>[2x]MYVCLCQGVTDNQI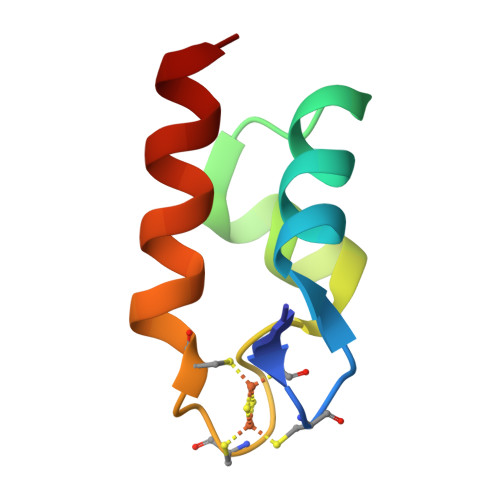RDAIYEGCCSYREVREATGVGTQCGKCASLAKQVVRETLNDL> GSPEFGALPVASPASLRTDLVKSELLHIESQVELLRFDDSGRKDSEVLKQNAVNSNQSNVVIEDFESSLTRSVPPLSQASLNIPGLPPEYLQVHLQESLGQEESQVSVTSADPVFQVPISKAVQLTTNDAIKTTLLVELDISNTDFS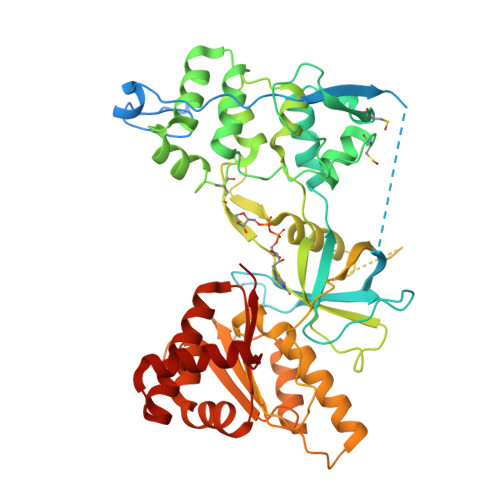YQPGDAFSVICPNSDSEVQSLLQRLQLEDKREHCVLLKIKADTKKKGATLPQHIPAGCSLQFIFTWCLEIRAIPKKAFLRALVDYTSDSAEKRRLQELCSKQGAADYSRFVRDACACLLDLLLAFPSCQPPLSLLLEHLPKLQPRPYSCASSSLFHPGKLHFVFNIVEFLSTATTEVLRKGVCTGWLALLVASVLQPNIHASHEDSGKALAPKISIFPRTTNSFHLPDDPSIPIIMVGPGTGIAPFIGFLQHREKLQEQHPDGNFGAMWLFFGCRHKDRDYLFRKELRHFLKHGILTHLKVSFSRDAPVGEEEAPAKYVQDNIQLHGQQVARILLQENGHIYVCGDAKNMAKDVHDALVQIISKEVGVEKLEAMKTLATLKEEKRYLQDIWS>[8x]EVSQDLFNQFNLFAQYSAAAYCGKNNDAPAGTNITCTGNACPEVEKADATFLYSFEDSGVGDVTGFLALDNTNKLIVLSFRGSRSIENWIG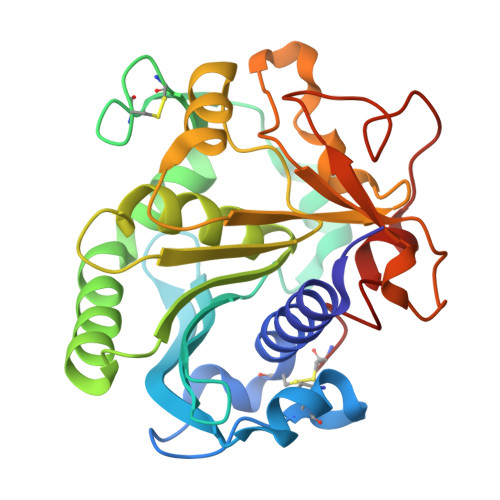NLNFDLKEINDICSGCRGHDGFTSSWRSVADTLRQKVEDAVREHPDYRVVFTGHSLGGALATVAGADLRGNGYDIDVFSYGAPRVGNRAFAEFLTVQTGGTLYRITHTNDIVPRLPPREFGYSHSSPEYWIKSGTLVPVTRNDIVKIEGIDATGGNNQPNIPDIPAHLWYFGLIGTCL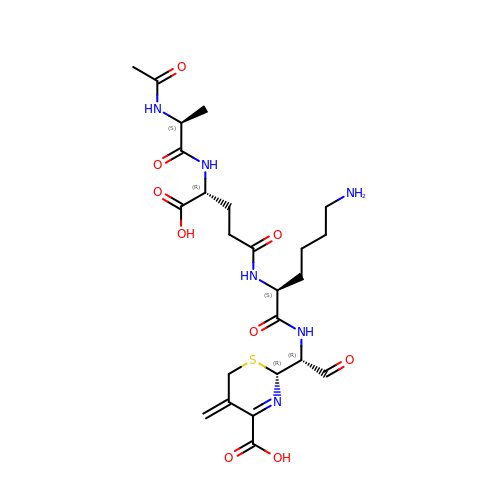2-(1-{2-[4-(2-ACETYLAMINO-PROPIONYLAMINO)-4-CARBOXY-BUTYRYLAMINO]-6-AMINO-HEXANOYLAMINO}-2-OXO-ETHYL)-5-METHYLENE-5,6-DIHYDRO-2H-[1,3]THIAZINE-4-CARBOXYLIC ACID | C24 H36 N6 O9 S | BZBLEHRBZDVRSG-JKCYHXNASA-N> VQQLSLFGSIGDDGYDLLISTLTTISGNPPLLYNSLCTVWKPNPSYDVENVNSRNQLVEPNRIKLSKEVPFSYLIDETMMDKPLNFRILKSFTNDKIPLNYAMTRNILHNTVPQVTNFNSTNEDQNNSKHTEDTVNESRNSDDIIDVDMDASPAPSNESCSPWSLQISDIPAAGNNRSVSMQTIAETIILSSAGKNSSVSSLMNGLGYVFEFQYLTIGVKFFMKHGLILELQKIWQIEEAGNSQITSGGFLLKAYINVSRGTDIDRINYTETVLMNLKKELQGYIELSVPDRQSMDS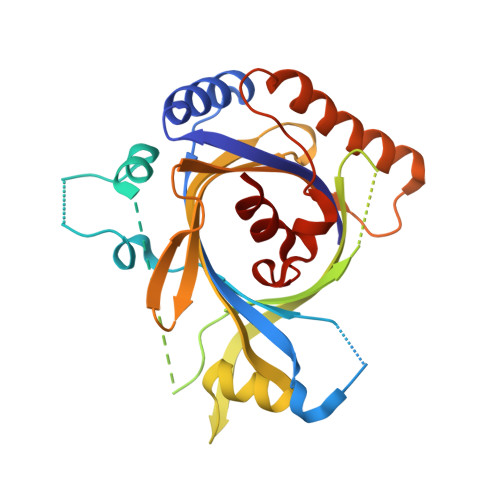RVAHGNILIAAALEHHHHHH>NQCLDVQSRDFVQGVSGGTWVDVVLDHDNCITIVADGKPSFDIRLSKMSMSKFAEYKRYCLQATMSDVTSIVACPGAGDAHNDKSKNHEYICKAVNNDRGWGNGCVLFGKGSMETCGKFECKKKMAGKLVARENVESVVTVHVHGASATDTKGVDTASTAKATITPKASVATLNLNDFGSLEVDCSTDVGMDFGEIVVADMSGKWWIVNKDWFNELALPWSTASTTAEVWQARDRLVEFGWPHAAKQNIYDIGDQEGAVTAAIAQAPMAKWESDKVELISGILKCKVKLGNLKLRGVTYSMCAQTFTTETRPADTGHGTVAFKVKYVGTDVPCRVPLHIIDSDGGVAAGRVITAHPFVMKQNDYIILEVEPPFGDSKIEIGTGTTKLVEAWHRKGSSIGNAFTATYKGITKLTVLGEHAWDFNSLGGFGASLGKAVHTLFGGVFRVMFGGMGWLTKIFVGAVLVWLGLGAHDKTIATTMILVGSILMYMAVTVGALS[3x];>ATLRTVGDLTWLNVSTTDVGKWIRVENRHGKGECFVTATDVGTWCSDSVGYECPQ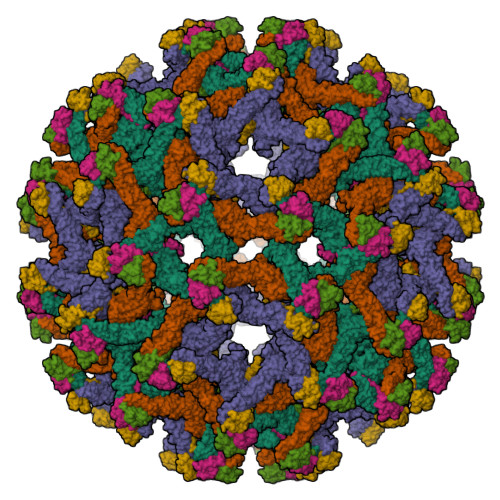IAPAYDPEDLDCYCRNTSTYVTYGRCKNGRSGRSRSKRAITIAPHGEAGLRVGSTKHWTSRATPQRYLMRVEKWVLRHPLPALVLVVLGWMMGRSHGQRAMYIVLMLLVAPSYG[3x]>MGHHHHHHMLHLLEQIRAYCETCWEWQEAHEPGMDQDKNPMPAPVEHQICPAVCVLMKLSFDEEHRHAMNELGGLQAIAELLQVDCEMYGLTNDHYSITLRRYAGMALTNLTFGDVANKATLCSMKGCMRALVAQLKSESEDLQQVIASVLRNLSWRADVNSKKTLREVGSVKALMECALEVKKESTLKSVLSALWNLSAHCTENKADICAVDGALAFLVGTLTYRSQTNTLAIIESGGGILRNVSSLIATNEDHRQILRENNCLQTLLQHLKSHSLTIVSNACGTLWNLSARNPKDQEALWDMGAVSMLKNLIHSKHKMIAMGSAAALRNLMANRPAKYKDANIMSPGSSLPS[6x];>PRDSYSGDALYEF[6x]

Adenomatous polyposis coli (APC) is an important human tumor suppressor protein which plays critical roles in diverse cellular processes such as Wnt/β-catenin signaling, cell adhesion, cell migration, mitosis and chromosomal instability, and so on. The N-terminal armadillo repeat (ARM) domain of APC is the most conserved region among its vertebrate and invertebrate homologs, and mediates its association with a variety of binding partners including APC membrane recruitment 1 (Amer1, also named as WTX for ‘Wilms tumor gene on the X chromosome’), Asef, Sam68, and IQGAP1. By recruiting APC to the plasma membrane, Amer1 regulates the APC-dependent maintenance of intercellular junctions. In addition, together with APC and Axin, Amer1 promotes ubiquitination and degradation of β-catenin, thus negatively regulates the Wnt signal transduction pathway.

Intriguingly, ITC experiments demonstrated that peptides of Amer1-A1 (residues 325–335) and -A2 (residues 496–508) sequences exhibited approximately equal binding affinities for APC–ARM as full Amer1-A1 (residues 280–368) and -A2 (residues 380–531), respectively. Therefore, Amer1 residues 325–335 and 496–508 are regarded to represent the core A1 and A2 fragments for APC binding, respectively, although other conserved Amer1 residues nearby such as residues 315–324 may also contribute to the interaction with APC. To further understand the molecular basis of how APC recognizes Amer1, we determined the crystal structures of the APC–ARM/Amer1-A1, APC–ARM/Amer1-A2, and APC–ARM/Amer1-A4 complexes to 1.90 Å, 2.00 Å, and 1.70 Å resolutions, respectively. Despite possessing apparently different sequences, Amer1-A1, -A2, and -A4 adopt remarkably similar conformations when bound to APC–ARM, both in anti-parallel manners with respect to the armadillo repeats of APC. In addition, two basic residues, APC-K516 and -R549, straddle the middle portion of Amer1-A1/A2/A4 peptides on both sides. They form salt bridges with a conserved acidic residue A1-D330/A2-D503/A4-E370 and make hydrogen bonds with the main chain carbonyl groups of A1-C328/A1-G329/A2-S501/A2-G502/A4-G368. Moreover, two tryptophan residues, APC-W593 and -W553, provide more binding affinity by hydrogen bonding with A1-T326/A2-S499 and making van der Waals interactions with A1-G327/A1-G329/A2-Y500/A2-G502/A4-G367/A4-G369, respectively. Accordingly, point mutations of T326R/T326A, D330K/D330A, and I332D in Amer1-A1 eliminated its binding with APC–ARM; the S499A, D503K/D503A, and L505D mutations in Amer1-A2 undermined its complex formation with APC–ARM; and the E370K point mutation or deletion of residues 370–373 in Amer1-A4 eliminated its interaction with APC–ARM. Moreover, the G329A mutation in Amer1-A1 and the D498K mutation in Amer1-A2 also attenuated their associations with APC–ARM as well.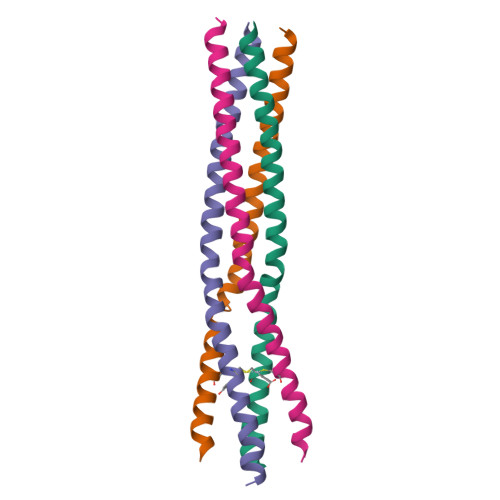>MLKKVEDTLTMLVNATSRQNAAIEALENRLSTLESSLKPIQDMGKVISSLNRSCAEMVAKYDLLEHHHHHH[4x]TDases are class A flavin-dependent monooxygenases that covalently modify and inactivate the core tetracycline moiety. Here, we investigate Tet(X6), a type 1 TDase first discovered in a Proteus genomospecies, by determining anhydrotetracycline-free and anhydrotetracycline-complexed X-ray crystal structures. Tet(X6) inactivates all classes of tetracyclines demonstrated by in vitro enzyme assays and phenotypic studies in E. coli. Here, we present structural, biochemical, and phenotypic evidence that anhydrotetracycline binds in a substrate-like orientation and competitively inhibits the type 1 TDase Tet(X6) to rescue tetracycline antibiotic activity as a sacrificial substrate.

An X-ray co-crystal structure of anhydrotetracycline in complex with Tet(X6) was determined at 2.2 Å resolution. A clear non-protein density was observed in the substrate-binding cavity, consistent with the size and shape of anhydrotetracycline. The anhydrotetracycline binds to Tet(X6) in a substrate-like orientation, placing the A-ring close to the FAD and the D-ring close to the C-terminal bridge helix. The isoalloxazine group of bound FAD occupies an ‘IN’ orientation in the Tet(X6)-anhydrotetracycline complex structure, as observed for the anhydrotetracycline-free structure. The carboxamide carbonyl oxygen at the 2-position of anhydrotetracycline forms a hydrogen bond with Arg213. A water molecule serves as a hydrogen-bonding bridge between the carboxamide substitution of anhydrotetracline and Thr59. In addition, the Phe224-side chain stabilizes the bound anhydrotetracycline through π-cation interaction with the 7-dimethylamino substitution of anhydrotetracycline. The O4 and N5 atoms of FAD form H-bonds to the keto-enol moiety (O12) and nearby hydroxyl group (O12a) of bound anhydrotetracycline. These interactions contribute to orienting the anhydrotetracycline scaffold for hydroxylation by a putative C4a-peroxy-flavin reactive intermediate at site C11a, with at an appropriate short distance of ~5.6 Å from the C4a of FAD-isoalloxazine heterocycle. The Tet(X6)-anhydrotetracycline complex shows the FAD cofactor bound in an ‘IN’ conformation that is distinct from the ‘OUT’ conformation observed for FAD in X-ray structures of type 2 TDases complexed with anhydrotetracycline.

>[2x]MTSSSHHHHHHSSGKLMTLKPANKNMTLLKHKKITIIGAGPVGLTMARLLQQNGVDITVYERDKDQDARIFGGTLDLHRDSGQEAMKRAGLLQTYYDLALPMGVNIVDEKGNILTTKNVRPENRFDNPEINRNDLRTILLNSLQNDTVIWDRKLVTLEPDKEKWILTFEDKSSETADLVIIANGGMSKVRKFVTDTEVEETGTFNIQADIHQPEVNCPGFFQLCNGNRLMAAHQGNLLFANPNNNGALHFGISFKTPDEWKSKTRVDFQDRNSVVDFLLKKFSDWDERYKELIRLTSSFVGLATRIFPLDKSWKSKRPLPITMIGDAAHLMPPFAGQGVNSGLMDALILSDNLTNGKFNSIEEAIENYEQQMFAYGREAQAESIINETEMFSLDFSFQKLMNL4-methyl-7-({3-[(methylamino)methyl]phenoxy}methyl)quinolin-2-amine | C19 H21 N3 O | 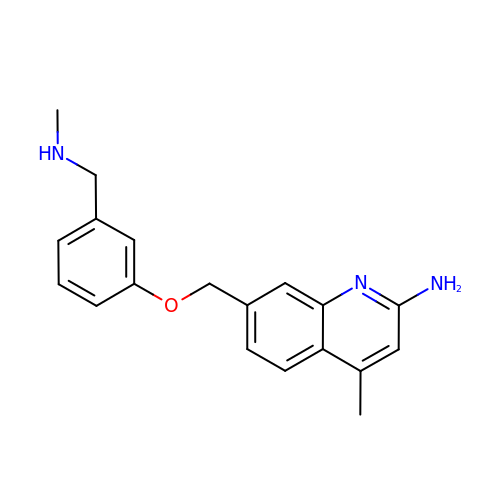XVIFXVGFIDKFPS-UHFFFAOYSA-N>PAGIIPTGNVLSTIEVCAHRCIFDFFKQIRSDDNSLYSAQFDILLGTYCNTLNFVRFLELGLSVACICTKFPELAYVRDGVIQFEVQQPMIARDGPHPVDQPVHNYMVKRIHKRSLSAAFAIASEALSLLSNTYVDGTEIDSSLRIRAIQQMARNLRTVLDSFERGTADQLLGVLLEKAPPLSLLSPINKFQPEGHLNRVARAALLSDLKRRVCADMFFMTRHAREPRLISAYLSDMVSCTQPSVMVSRITHTNTRGRQVDGVLVTTATLKRQLLQGILQIDDTAADVPVTYGEMVLQGTNLVTALVMGKAVRGMDDVARHLLDITDPNTLNIPSIPPQSNSDSTTAGLPVNARVPADLVIVGDKLVFLEALERRVYQATRVAYPLIGNIDITFIMPMGVFQANSMDRYTRHAGDFSTVSEQDPRQFPPQGIFFYNKDGILTQLTLRDAMGTICHSSLLDVEATLVALRQQHLDRQCYFGVYVAEGTEDTLDVQMGRFMETWADMMPHHPHWVNEHLTILQFIAPSNPRLRFELNPAFDFFVAPGDVDLPGPQRPPEAMPTVNATLRIINGNIPVPLCPISFRDCRGTQLGLGRHTMTPATIKAVKDTFEDRAYPTIFYMLEAVIHGNERNFCALLRLLTQCIRGYWEQSHRVAFVNNFHMLMYITTYLGNGELPEVCINIYRDLLQHVRALRQTITDFTIQGEGHNGETSEALNNILTDDTFIAPILWDCDALIYRDEAARDRLPAIRVSGRNGYQALHFVDMAGHNFQRRDNVLIHGRPVRGDTGQAIPITPHHDREWGILSKIYYYIVIPAFSRGSCCTMGVRYDRLYPALQAVIVPEIPADEEAPTTPEDPRHPLHAHQLVPNSLNVYFHNAHLTVDGDALLTLQELMGDMAERTTAILVSSAPDAGAATATTRNMRIYDGALYHGLIMMAYQAYDETIATGTFFYPVPVNPLFACPEHLASLRGMTNARRVLAKMVPPIPPFLGANHHATIRQPVAYHVTHSKSDFNTLTYSLLGGYFKFTPISLTHQLRTGFHPGIAFTVVRQDRFATEQLLYAERASESYFVGQIQVHHHDAIGGVNFTLTQPRAHVDLGVGYTAVCATAALRCPLTDMGNTAQNLFFSRGGVPMLHDNVTESLRRITASGGRLNPTEPLPIFGGLRPATSAGIARGQASVCEFVAMPVSTDLQYFRTACNPRGRASGMLYMGDRDADIEAIMFDHTQSDVAYTDRATLNPWASQKHSYGDRLYNGTYNLTGASPIYSPCFKFFTPAEVNTNCNTLDRLLMEAKAVASQSSTDTEYQFKRPPGSTEMTQDPCGLFQEAYPPLCSSDAAMLRTAHAGETGADEVHLAQYLIRDASPLRGCLPL[6x];>SNPTTFSVEAIAAYTPVALIRLLNASGPLQPGHRVDIADARSIYTVGAAASAARARANHNANTIRRTAMFAETDPMTWLRPTVGLRRTFNPRII[6x];>AMPFEIEVLLPGELSPAETSALQKCEGKIITFSTLRHRASLVDIALSSYYINGAPPDTLSLLEAYRMRFAAVITRVIPGK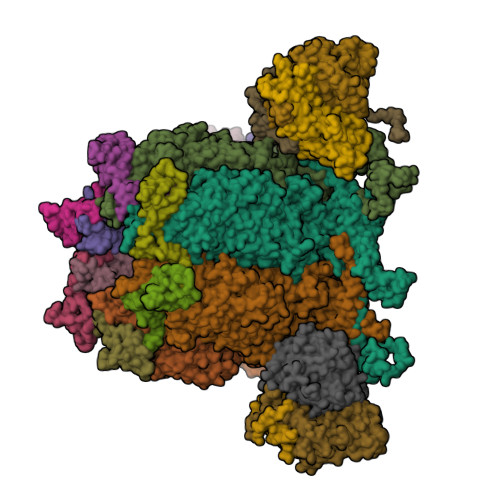LLAHAIGVGTPTPGLFIQNTSPVDLCNGDYICLLPPVYGSADSIRLDSVGLEIVFPLTIPQTLMREIIAKVVARAVEDLNLMFSINEGCLLILALIPRLLALLIPRLLALVTREAAQLIHPEAPMLMLPIYETISSWISTSSRLGDTLGTRAILRVCVFDGPSTVHPGDRTAVIQV[2x];>AMPFEIEVLLPGEISPAETSALQKCEGKIITFSTLRHRASLVDIALSSYYINGAPPDTLSLLEAYRMRFAAVITRVIPGKLLAHAIGVGTPTPGLFIQNTSPVDLCNGDYICLLPPVFGSADEIRLDSVGLEIVFPLTIPQTLMREIIAKVVARAVERTAADVICYNGRRYELETNLQHRDGSDAAIRTLVLNLMFSINEGTTLILTLITRLLRFPIYEAISSWISTSSRLGDTLGTRAILRVCVFDGPSTVHPGDRTAVIQV[2x];>AAAAAAAAAAAAAAAAAAAAFKSTTQLIQQVSLTDFFRPDIEHAGSTVLILRHPTDLPALARHRAPPGRQTERLAEAWGQLLEASRAYVTSLSFIAACRAEEYTDKQAAEANRTAIVSAYGCSRMGARLIRFSECLRAMVQCHVFPHRFISFFGSLLEYTIQDNLCNITAVAKGPQEAARTDKTSTRRVTANIPACVFWDVDKDLHLSADGLKHVFLVFVYTQRRQREGVRLHLALSQLNEQCFGRGIGFLLGARICMYAAYTLIGTIPSESVRYTRRMERFGGYNVPTIWLEGVVWGGTNTWNEC[2x]> MNVTVDQSTLAGATRGIVRGGETLKEHRDRLMAATKATGRYAGLKTLELREREPILYNKLFSRLRAGVVDARETAKKIAASPIVEQEGELCFTLYNAAGDSLLTSTGIIIHVGTMGAAIKYMIENNWEANPGVHDKDIFCNNDSLIGNVHPCDIHTIVPIFWEGELIGWVGGVTHVIDTGAVGPGSMATGQVQRFGDGYSITCRKVGANDTLFRDWLHESQRMVRTTRYWMLDERTRIAGCHMIRKLVEEVVAEEGIEAYWKFAYEAVEHGRLGLQARIKAMTIPGTYRQVGFVDVPYAHEDVRVPSDFAKLDTIMHAPCEMTIRRDGTWRLDFEGSSRWGWHTYNAHQVSFTSGIWVMMTQTLIPSEMINDGAAYGTEFRLPKGTWMNPDDRRVAFSYSWHFLVSAWTALWRGLSRSYFGRGYLEEVNAGNANTSNWLQGGGFNQYDEIHAVNSF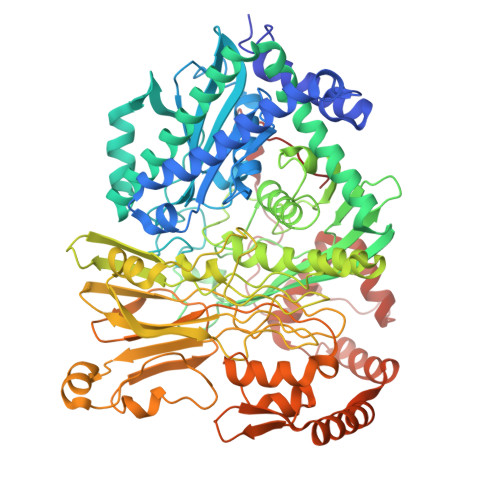ECAANGTGATAVQDGLSHAAAIWNPEGDMGDMEIWELAEPLVYLGRQIKASSGGSGKYRGGCGFESLRMVWNAKDWTMFFMGNGHISSDWGLMGGYPAASGYRFAAHKTNLKELIASGAEIPLGGDTDPENPTWDAMLPDAQIKRDKQAITTEEMFSDYDLYLNYMRGGPGFGDPLDREPQAVADDINGGYVLERFAGEVYGVVVRKGADGQYGVDETATAAARAQIRKDRLAKSVPVSEWMKGEREKILAKDAGTQVRQMFAASFKLGPRFEKDFRTFWDLPDSWTLPEEEIGVPTYGSRYSMDISELPDVHTVQFVEE>MIRTMLQGKLHRVKVTHADLHYEGSCAIDQDFLDAAGILENEAIDIWNVTNGKRFSTYAIAAERGSRIISVNGAAAHCASVGDIVIIASFVTMPDEEAR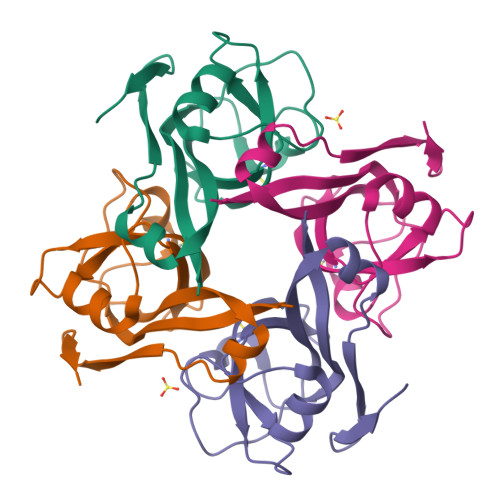TWRPNVAYFEGDNEMKRTAKAIPVQVA[2x]> MSTRPEVFDLIVIGGGPGGSTLASFVAMRGHRVLLLEREAFPRHQIGESLLPATVHGICAMLGLTDEMKRAGFPIKRGGTFRWGKEPEPWTFGFTRHPDDPYGFAYQVERARFDDMLLRNSERKGVDVRERHEVIDVLFEGERAVGVRYRNTEGVELMAHARFIVDASGNRTRVSQAVGERVYSRFFQNVA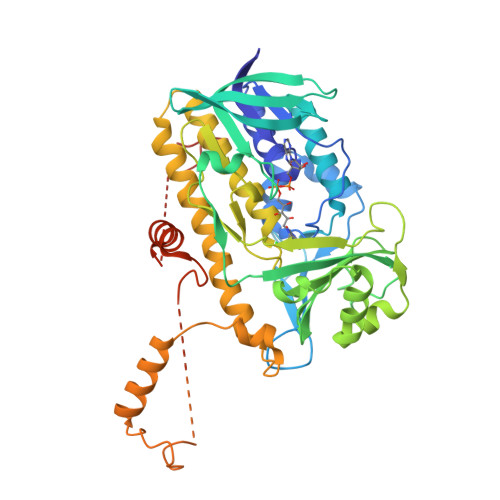LYGYFENGKRLPAPRQGNILSAAFQDGWFWYIPLSDTLTSVGAVVSREAAEAIKDGHEAALLRYIDRCPIIKEYLAPATRVTTGDYGEIRIRKDYSYCNTSFWKNGMALVGDAACFVDPVFSSGVHLATYSALLVARAINTCLAGEMSEQRCFEEFERRYRREYGNFYQFLVAFYDMNQDTDSYFWSARKIINTEERANEAFVRLIAGRSNLDEPVFQSVAKDFFTEREGFGAWFGGLVTSMAKGDGGGLMVGEGATDATESTGFAPENFMQGFTREITELQHLAMFGEDRGPETPLWSGGLVPSRDGLAWAVESGEDAAG> SSQEYAYIDVDI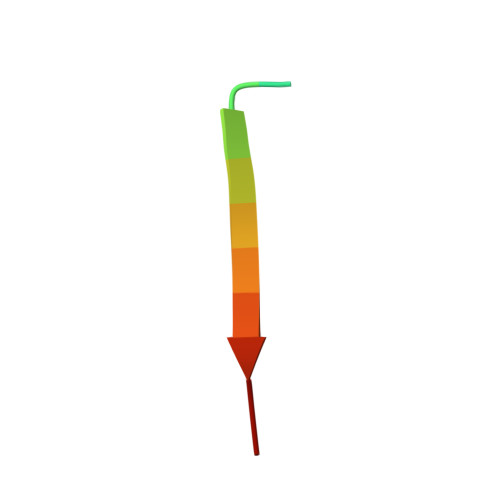N> GSSGSSGMRLNVNPTRMELTRLKKQLTTATRGHKLLKDKQDELMRQFILLIRKNNELRQAIEKETQTAMKDFVLAKSTVEEAFIDELLALPAENVSISVVEKNIMSVKVPLMNFQYDETLNETPLEYGYLHSNAELDRSIDGFTQLLPKLLKLAEVEKTCQLMA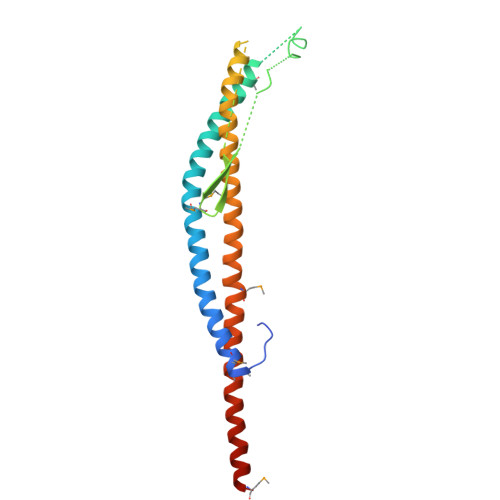EEIEKTRRRVNALEYMTIPQLEETIYYIKMKLEENERAEVTRLIKVKNMGTEE{(1R)-3-oxo-1-phenyl-3-[4-(trifluoromethyl)phenyl]propyl}propanedioic acid | 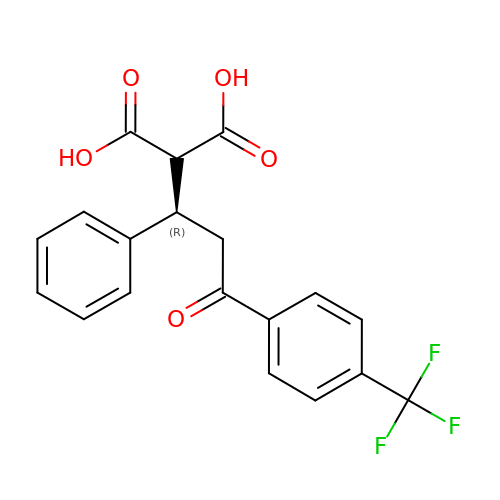C19 H15 F3 O5 | MLJPLHGJBUWCBA-AWEZNQCLSA-N>GPTSHHFCFSIDLRSIHALEIGFPINCILRYSYPFFGSAAPIMTNPPVEVRKNMEVFLPQSYCAFDFATMPHQLQDTFLRIPL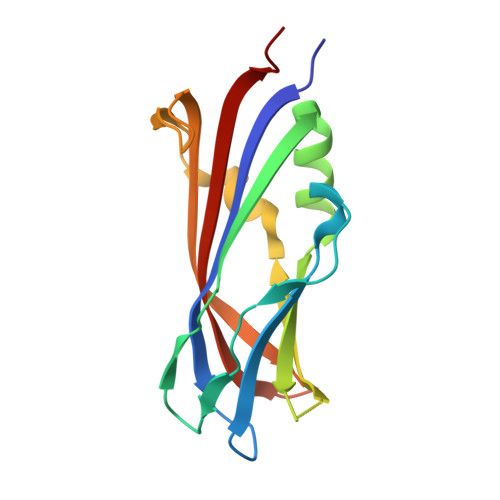LVELWHKDKMSKDLLLGIARIQLSNILSSEKTRFLGSNGEQCWRQTYSESVPVIAAQGSNNRIADLSYTVTLEDYGLVKM[2x]> SNPFAHLAEPLDPVQPGKKFFNLNKLEDSRYGRLPFSIRVLLEAAIRNCDEFLVKKQDIENILHWNVTQHKNIEVPFKPARVILQDFTGVPAVVDFAAMRDAVKKLGGDPEKINPVCPADLVIDHSIQVDFNRRADSLQKNQDLEFERNRERFEFLKWGSQAFHNMRIIPPGSGIIHQVNLEYLARVVFDQDGYYYPDSLVGTDSHTTMIDGLGILGWGVGGIEAEAVMLGQPISMVLPQVIGYRLMGKPHPLVTSTDIVLTITKHLRQVGVVGKFVEFFGPGVAQLSIADRATIANMCPEYGATAAFFPVDEVSITYLVQTGRDEEKLKYIKKYLQAVGMFRDFNDPSQDPDFTQVVELDLKTVVPCCSGPKRPQDKVAVSDMKKDFESCLGAKQGFKGFQVAPEHHNDHKTFIYDNTEFTLAHGSVVIAAITSCTNTSNPSVMLGAGLLAKKAVDAGLNVMPYIKTSLSPGSGVVTYYLQESGVMPYLSQLGFDVVGYGCMTCIGNSGPLPEPVVEAITQGDLVAVGVLSGNRNFEGRVHPNTRANYLASPPLVIAYAIAGTIRIDFEKEPLGVNAKGQQVFLKDIWPTRDEIQAVERQYVIPGMFKEVYQKIETVNESWNALATPSDKLFFWNSKSTYIKSPPFFENLTLDLQPPKSIVDAYVLLNLGDSVTTDHISPAGNIARNSPAARYLTNRGLTPREFNSYGSRRGNDAVMARGTFANIRLLNRFLNKQAPQTIHLPSGEILDVFDAAERYQQAGLPLIVLAGKE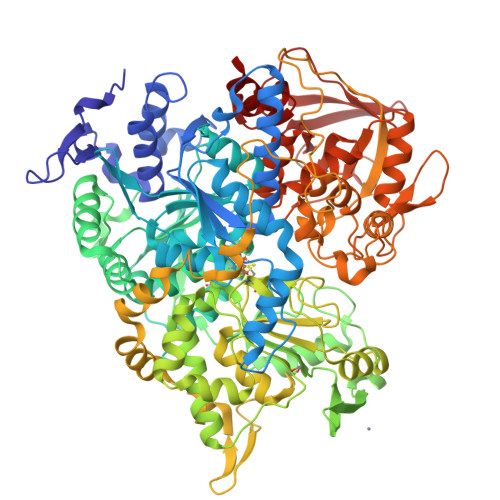YGAGSSRDWAAKGPFLLGIKAVLAESYERIHRSNLVGMGVIPLEYLPGENADALGLTGQERYTIIIPENLKPQMKVQVKLDTGKTFQAVMRFDTDVELTYFLNGGILNYMIRKMAK The TP901-1 switch is encoded by a < 1 kb fragment of the phage genome, including genes for the CI repressor and a Mor (modulator of repression) antirepressor (transcribed from the PR and PL promotors, respectively) instead of Cro. As for phage λ, CI in TP901-1 contains a DNA-binding, N-terminal domain (CI-NTD), which consists of a characteristic helix-turn-helix (HTH) structure. Cooperative binding of the TP901-1 CI dimer to OL ensures maintenance of the lysogenic, immune state, and inhibition of expression of lytic genes and mor. Structural evidence from a CI-NTD:Mor complex and a CI-NTD:DNA complex strongly suggests that it functions as an antirepressor by steric hindrance, preventing binding of CI-NTD monomers in a dimer to adjacent half-sites on OL.

However, none of the uncomplexed structures of CI-NTD corresponded to the identical sequence of the construct used for the interaction studies with Mor, which motivated a new crystallization effort. The new X-ray structure, which has by far the highest resolution for a TP901-1 CI-NTD structure obtained so far, resembles the overall previous structures of TP901-1 CI-NTD with the typical HTH motif. Generally, the structure is of high quality. It was determined at a maximum resolution of 1.29 Å with a final R factor of 14.97% and R free of 18.29%. However, several exposed side chains have alternate conformations (Met1, Ser6, Gln11, Ile12, Met13, Glu15, Ile23, Ser41, Ser44, Ile58, Glu69, Met73, Met79, and Val80) or are not fully visible in the electron density maps. However, there was definite disordered electron density beyond this point, which, after many attempts, was modeled as res 81 connected to the rest of the chain and two additional residues (83-84) after a one-residue gap. As modeled, the positions of res 81 and the res 83-84 segment are not compatible with each other, but each represents one of presumably multiple conformations assumed by the chain in this area. Gln55, Glu69, and Met73 (underlined in the sequences above) stand out as interface residues taking on different conformations in different crystal structures. In the most recent high-resolution structure, there are no such interactions and two conformations were necessary for adequate modeling of the side chain. An omit map where Glu69 was modeled as Ala clearly indicates that the Glu69 side chain density would clash with Phe67 of Mor in the complex; thus, a considerable rearrangement is required on complex formation. Instead, the most notable rearrangement upon complex formation is Glu69, which forms an unusual interaction with the aromatic ring of Phe67 in Mor through its aliphatic chain.

> MQTDTSNRLKQIMAERNLKQVDILNLSIPFQKKFGIKLSKSTLSQYVNSVQSPDQNRIYLLAKTLGVSEAWLMGFDVPMVESSKIENDSHHHHHH> GPLGSSQIPASEQETLVRPKPLLLKLLKSVGAQKDTYTMKEVLFYLGQYIMTKRLYDAAQQHIVYCSNDLLGD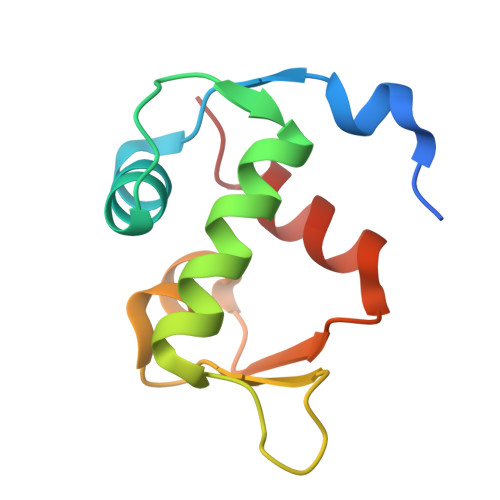LFGVPSFSVKEHRKIYTMIYRNLV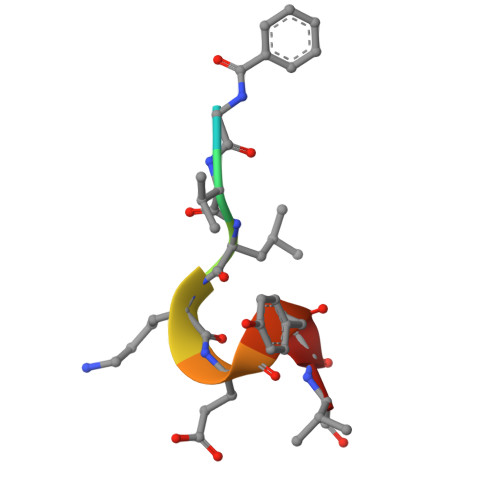> XGVLKEYGV>[2x]HHHHHHGSERTGTQP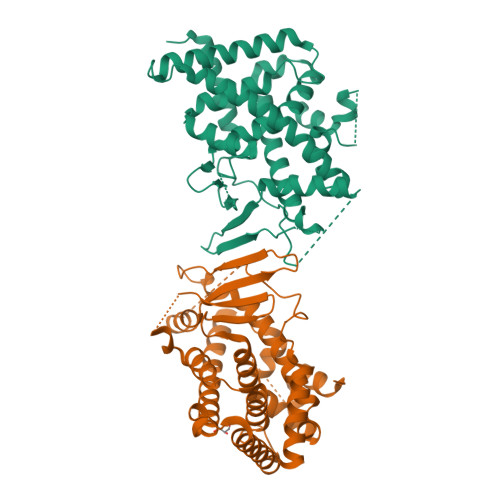LGVQGLTEEQRMMIRELMDAQMKTFDTTFSHFKNFRLPGVLSSGCELPESLQAPSREEAAKWSQVRKDLCSLKVSLQLRGEDGSVWNYKPPADSGGKEIFSLLPHMADMSTYMFKGIISFAKVISYFRDLPIEDQISLLKGAAFELCQLRFNTVFNAETGTWECGRLSYCLEDTAGGFQQLLLEPMLKFHYMLKKLQLHEEEYVLMQAISLFSPDRPGVLQHRVVDQLQEQFAITLKSYIECNRPQPAHRFLFLKIMAMLTELRSINAQHTQRLLRIQDIHPFATPLMQEVFGITGSSGGSGGSSHSSLTERHKILHRLLQEGSPSDITTLSVEPD> GVTFDDGAYTGIREINFEYNSETAIGGLRVTYDLNGMPFVAEDHKSFITGFKPVKISLEFPSEYIVEVSGYVGKVEGYTVIRSLTF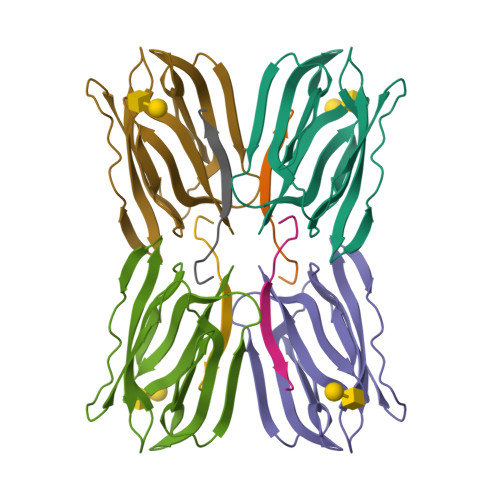KTNKQTYGPYGVTNGTPFSLPIENGLIVGFKGSIGYWLDYFSIYLSL;> NGKSQSIIVGPWGD> MHHHHHHSSGRENLYFQGTFAERYNIVCMLGKGSFGE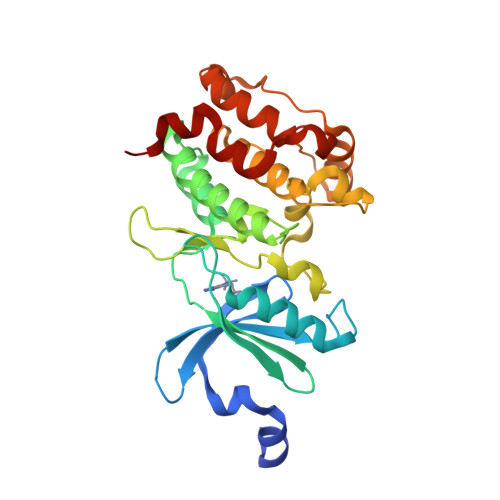VLKCKDRITQQEYAVKVINKASAKNKDTSTILREVELLKKLDHPNIMKLFEILEDSSSFYIVGELYTGGELFDEIIKRKRFSEHDAARIIKQVFSGITYMHKHNIVHRDLKPENILLESKEKDCDIKIIDFGLSTCFQQNTKMKDRIGTAYYIAPEVLRGTYDEKCDVWSAGVILYILLSGTPPFYGKNEYDILKRVETGKYAFDLPQWRTISDDAKDLIRKMLTFHPSLRITATQCLEHPWIQKYSSEE>[2x]HTSPLLAPVRQIHAFGDXYSDNGESQRLTREMLAKGIAGAQALPGEVYWQGRWSNGPTAVEVLA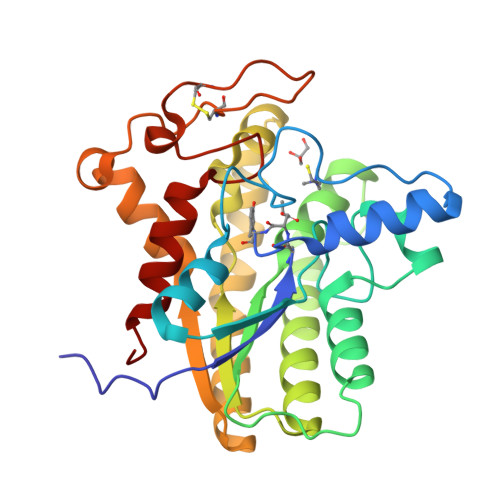RQLGAQLADHAVGGAKSGADNYYGWMSAYRHTGLAGQVDAYLATLDGKPVDGQALHFIFVSANDFFEHEDFAGEQPLEQLAGSSVANIRAAVQRLGEAGARRFLVVSSTDLSVVPAVVAGNRVERAQRYLQAVNASLPIQLAALRKTRGLELSWFDHLTFSRHLRRNPARYGLVELDAPCQPTQPSVRPACANPDQYYFWNEWHPTRRVHQLAGEAMAARYAR[cyclohexyl(hydroxy)amino](oxo)acetic acid | C8 H13 N O4 | 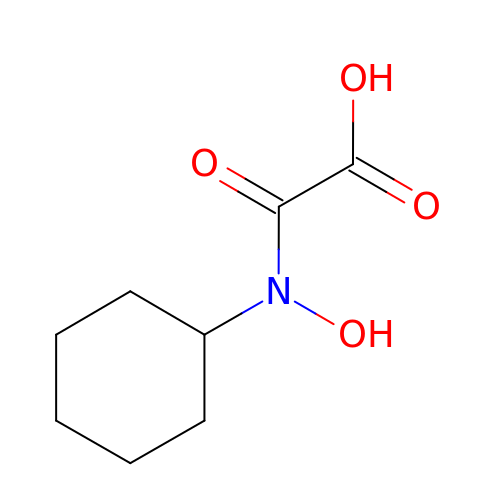HMDGECZILRJLEV-UHFFFAOYSA-N>VSHVQSSASVPGLIELLESNTIFGNEAELLEKEGLSINYPNCRSWHLGVETSNIINFDTVPANCKAYVEDYLITSKQYQYD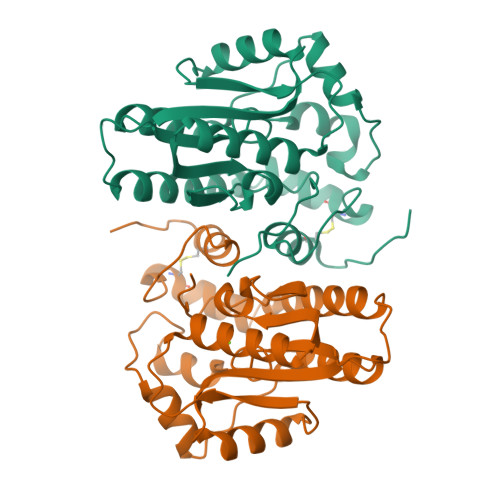SKTVNKEAYFYAKGLALKNDTVNVWIFDLDDTLLSSIPYYAKYGYGTENTAPGAYWSWLESGESTPGLPETLHLYENLLELGIEPIIISDRWKKLSEVTVENLKAVGVTKWKHLILKPNGSKLTQVVYKSKVRNSLVKKGYNIVGNIGDQWADLVEDTPGRVFKLPNPLYYVPSLEHHHHHH[2x]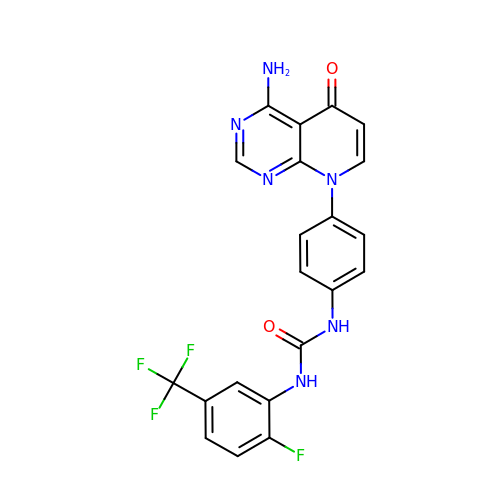1-[4-(4-amino-5-oxopyrido[2,3-d]pyrimidin-8(5H)-yl)phenyl]-3-[2-fluoro-5-(trifluoromethyl)phenyl]urea | C21 H14 F4 N6 O2 | OWKPAZCWJGPSQU-UHFFFAOYSA-N>[6x]GPMSFLFG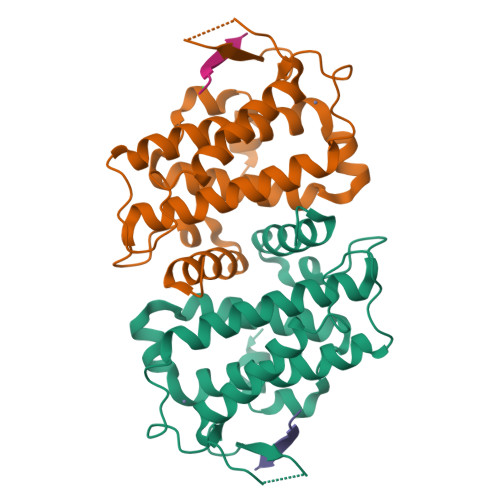SRSSKTFKPKKNIPEGSHQYELLKHAEATLGSGNLRMAVMLPEGEDLNEWVAVNTVDFFNQINMLYGTITDFCTEESCPVMSAGPKYEYHWADGTNIKKPIKCSAPKYIDYLMTWVQDQLDDETLFPSKIGVPFPKNFMSVAKTILKRLFRVYAHIYHQHFDPVIQLQEEAHLNTSFKHFIFFVQEFNLIDRRELAPLQELIEKLTSKDR> MKN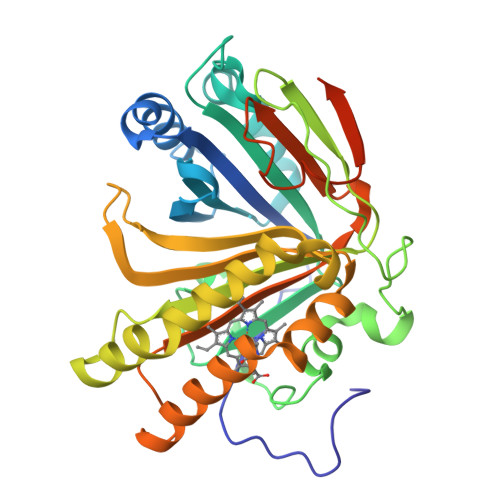MPENHNPQANAWTAEFPPEMSYVVFAQIGIQSKSLDHAAEHLGMMKKSFDLRTGPKHVDRALHQGADGYQDSIFLAYWDEPATFKSWVADPEVQKWWSGKKIDENSPIGYWSEVTTIPIDHFETLHSGENYDNGVSHFVPIKHTEVHEYWGAMRDRMPVSASSDLESPLGLQLPEPIVRESFGKRLKVTAPDNICLIRTAQNWSKCGSGERETYIGLVEPTLIKANTFLRENASETGCISSKLVYEQTHDGEIVDKSCVIGYYLSMGHLERWTHDHPTHKAIYGTFYEMLKRHDFKTELALWHEVSVLQSKDIELIYVNCHPSTGFLPFFEVTEIQEPLLKSPSVRIQKLAAALEHHHHHH>GPGMDNNVSQEMTVPVEGVAGGGTAYGFNDAEPLKQSTDPSEVPTADLVNVWCMPNTVNVGSQETPRALEPINLLAARNERESFQIAMRPKVSWAASSPSGIVQVQCSDLCSSAGDRLVVGQSLKLRRVVPVLGVPDALVPLDLPVSQLSLFPGETSVIWVSIDVPTGQPPGQYEGEIIISAMKTDGGGSSHLAKHEKDQLCVELNTCLDIMEPIEGKPMDEVVERIKCASSSLRRILFSPSFSEFISTNGSTDMMEEDVVSNLSLRIKLRLTVWEFIIPVTPSLPAVIGVSDTVIEDRFAVEHGSEDWYKKLDLHFKWLLQYRISPYFCKWGESMRVLTYTSPWPADHPKSDEYLSDSRLAAYAVPYRQVIAGDDSRESYLRKEVEILRSKPHWNKAYFYLWDEPLNMEHFDNVRKMASEIYAYAPDSRVLTTYYCGPGDAPLAPTPFESFVKVPNLLRPYTQIYCTSEWVLGNREDLVKDILDELQTENGEEWWTYICLGPSDPHPNWHLGMRGTQQRAVMWRVWKEGGTGFLYWGANCYEKATVPSAEVKFRRGLPPGDGVLYYPGEVFSSSSEPVASLRLERLLSGLQDYEYLKLYESKYGREEAMGLLEKTGVYTGPERYTLEHRPIDVLRGEVYNTCRPS[2x]

Beta-N-acetylgalactosaminidases (β-NGAs) hydrolyze the different β-GalNAc linkages of various glycans to modulate the length, combination, and abundance of glycans. Despite low sequence similarity, the crystal structures of these enzymes demonstrate that all enzymes share a prototype structure and have diversified their substrate specificities (oligosaccharide-releasing, oligosaccharide/monosaccharide-releasing, and monosaccharide-releasing) through the accumulation of mutations and insertional amino acid sequences. The overall structure of these enzymes is similar to that of CpNga123 and BvGH123, which consist of a β-sandwich domain at the N-terminus and a (β/α)8-barrel domain encompassing the catalytic region. Among Groups 1–4 and GH123, the DE motif is located at the same position, suggesting that these enzymes adopt the substrate-assisted catalysis reported for GH123 MR-β-NGAs.

In Group 2, NgaAt was active against GalNAc-β-pNP and GlcNAc-β-pNP but not against Galβ1-3GalNAc-β-pNP, indicating that it possessed MR-β-HEX activity. Thus, NgaAt is a different linage of β-HEX from GH20. Among the enzymes identified herein, only NgaAt (Group 2) is a β-HEX that acts on β-GalNAc and β-GlcNAc [NgaAt (locus_tag = AT1G45150) is currently annotated as an α-1,6-mannosyl-glycoprotein 2-beta-N-acetylglucosaminyltransferase (EC 2.4.1.143); this annotation needs correcting based on our findings]. The active site of NgaAt in Group 2 also possesses a cleft shape, and the second β-sheet of the (β/α)8 barrel is longer than that found in the other enzymes, followed by an additional β-sheet (orange). Thus, NgaAt demonstrates more diverse activity than expected and possesses OR/MR-β-HEX functionality. NgaAt was inhibited by 25 nM GalNAc-thiazoline and by 25 μM GlcNAc-thiazoline (a 1000-fold higher concentration) (orange and yellow). The increased number of residues could potentially reinforce substrate recognition in Group 4 and GH123 enzymes. Additional structural analyses (comparison of crystal structure with AlphaFold2 predicted structure of NgaCa, comparison of apo1-form and apo2-form of NgaCa, and comparison of GalNAc-thiazoline-bond form and GlcNAc-thiazoline-/apo-form of NgaAt, NgaDssm, and NgaP2) data are illustrated in Supplementary Fig. 13. The structure of NgaDssm (Group 3) bore a striking resemblance to that of NgaLy and NgaP2 (Group 4) (root-mean-square distance of Cα atoms [rmsd] = 1.5–2.3 Å), while the structures of NgaLy and NgaP2 are identical (rmsd = 1.0 Å). The additional N-terminal domain consisting of ~80 amino acids, found only in Group 2 enzymes, was not modeled in the crystal structure of NgaAt owing to disorder (orange circle).2-(BETA-D-GLUCOPYRANOSYL)-5-METHYL-1-BENZIMIDAZOLE | 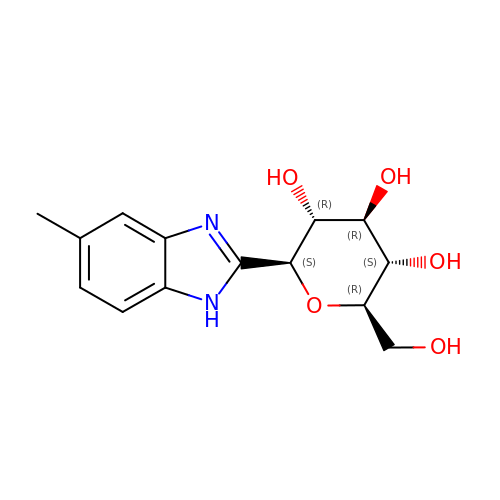C14 H18 N2 O5 | XIJZORUYQZBFJK-UJPOAAIJSA-N> GSILAETHGTRPDLT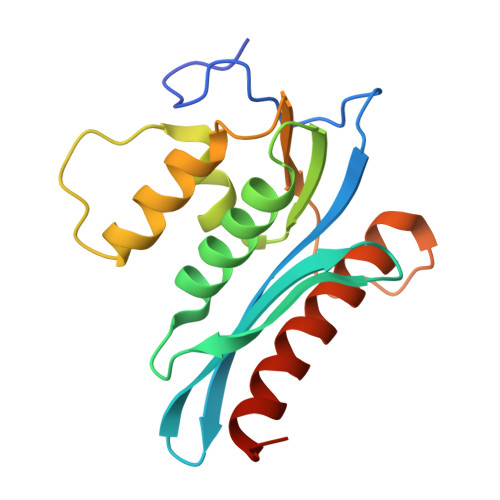DQPIPDADYTWYTDGSSFLQEGQRRAGAAVTTETEVIWARALPAGTSAQRAELIALTQALKMAEGKKLNVYTDSRYAFATAHVHSEGREIKNKNEILALLKALFLPKRLSIIHCPGHQKGNSAEARGNRMADQAAREAAMKAVLETSTLL>GSSHHHHHHSSGLVPRGSHMASAQETTRLTATEIRARISEGAASREEVVHEHLDRIDEFNALTNSFVELRADQVLEEARAADREFGSTLGGPLDGVPLSIKDSYSVAGLHRTDGLPVNADVLDAQDDVATARLRAAGGLVLGHAGIPDLCIRWNSVSGLYGAVRNPRDLSRTAGGSSGGDAANVAAGFATIGLGGDLGGSIRVPASWCGVYGFRTGPGRIPDVNPNGGRSRNVVMELMAQIGPIARSIDDIELAFRIMTGVDRRDTMSSPLGLIEPIEAPRVAVLRHETGAVLDSSVEEQLDATIEMLRAEGYVVEENVLPDLHRAPEVWAEIVGTELIHRVLPEVAELVIASERMHIVDMFGAYELGADVGAYLTALEERSSIQMTVAALMERYQLILAPVAGMPAPPLDFDDHIGREASIALFDQMRCVPWVNLLGLPSLALPNGIQLVGRKHDELTILAAGRAY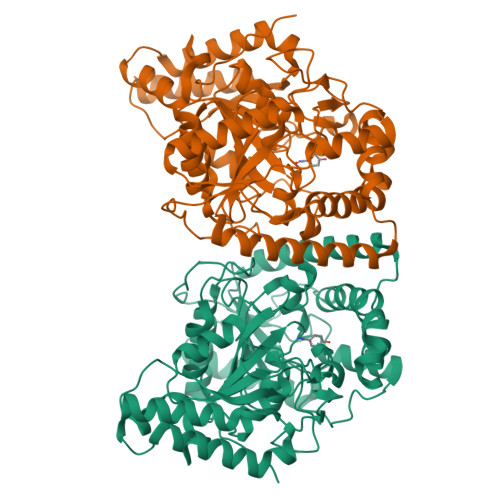ERRAPRVEIATPAI[4x]> GSHMKPRGKRGWLWLLLKLAIVFAVLIAIYGVYLDQKIRSRIDGKVWQLPAAVYGRMVNLEPDMTISKNEMVKLLEATQYRQVSKMTRPGEFTVQANSIEMIRRPFDFPDSKEGQVRARLTFDGDHLATIVNMENNRQFGFFRLDPRLITMISSPNGEQRLFVPRSGFPDLLVDTLLATEDRHFYEHDGISLYSIGRAVLANLTAGRTVQGASTLTQQLVKNLFLSSERSYWRKANEAYMALIMDARYSKDRILELYMNEVYLGQSGDNEIRGFPLASLYYFGRPVEELSLDQQALLVGMVKGASIYNPWRNPKLALERRNLVLRLLQQQQIIDQELYDMLSARPLGVQPRGGVISPQPAFMQLVRQELQAKLGDKVKDLSGVKIFTTFDSVAQDAAEKAAVEGIPALKKQRKLSDLETAIVVVDRFSGEVRAMVGGSEPQFAGYNRAMQARRSIGSLAKPATYLTALSQPKIYRLNTWIADAPIALRQPNGQVWSPQNDDRRYSESGRVMLVDALTRSMNVPTVNLGMALGLPAVTETWI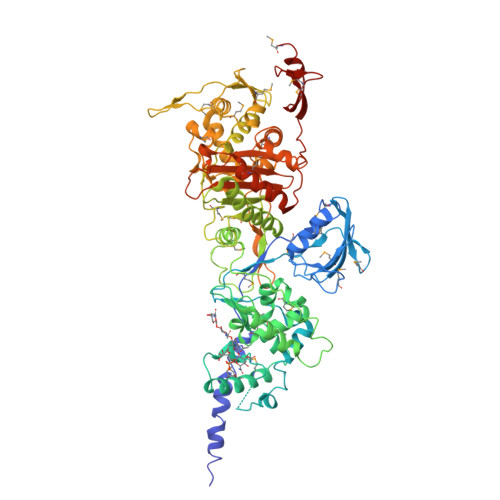KLGVPKDQLHPVPAMLLGALNLTPIEVAQAFQTIASGGNRAPLSALRSVIAEDGKVLYQSFPQAERAVPAQAAYLTLWTMQQVVQRGTGRQLGAKYPNLHLAGKTGTTNNNVDTWFAGIDGSTVTITWVGRDNNQPTKLYGASGAMSIYQRYLANQTPTPLNLVPPEDIADMGVDYDGNFVCSGGMRILPVWTSDPQSLCQQSEMQQQPS>[2x]GPLGSMEGFERELDNIPDTLPDDERLALWKGKLKHYLILSSAGKPIWSRHGDLSLVNSTMGVVQTIISFYEGARNPLLGFTAGKVRFVILIKGPLYFVAISRLRESDAQLRAQLEALYMQILSTLTLPILTNIFAHRPSTDLRGPLQGTESLLASLADSFTKGSPS;>SMTTPVSPSPSGIIPAQLGFLAIYNPALGTTDETLEDQIVYYATASTLSQARRRHRRPRRRDRQRAQSVVKDSRPNAAGATGDSEAVAEDKDPVSKEERHERLRQIGLAQGMVEFAKSFSDGEPVDTIDTEKARVILVEVEEGWWILASIDLTRLPLPQIKTPTSSSAPPPAPNLNPLPPEPAYEYSSREVKPPSLLRADLLRAYDLFLLHHGSSLSSLLASQGRAQLVASLTRFWDHFLATWNVLLHGN[2x];>[2x]GSMSSRKKVLLKVIILGDSGVGKTSLMNQYVNKKFSASYKATIGADFLTREVMVDDRQVTMQLWDTAGQERFQSLGVAFYRGADCCVLVFDVNNAKSFDALDSWRDEFLIQASPRDPENFPFVVLGIKIDVEESKRVISTKRAQTFCQSKGGIPYFETSAKEAINVEEAFQVIARNALMQEESEEFSGDFQDPINIHIENERDGCAC

MC1 has been identified as the GEF for Rab7/Ypt7 and localizes to LEs1216. The sequential inactivation of Rab5 and activation of Rab7 (Ypt7 in yeast), which then serves as marker for LEs, confers membrane identity and directionality during the endosomal maturation process26. Our study shows that MC1 forms a heterotetrameric complex with specific localization domains and a catalytic core that acts through a unique mechanism, thus representing a novel class of RabGEFs. The enzymatic activity of MC1 is mediated entirely by a core complex consisting of the longin domains of Mon1 and Ccz1 plus an extra N-terminal helix of Mon1.

To gain mechanistic insight into MC1 function, we determined the crystal structure of the catalytically active CtMC1core bound to the nucleotide-free CtYpt7–N125I. The structure was refined to 2.5 Å resolution revealing two CtMC1–Ypt7 complexes per asymmetric unit. Mon1 as well as Ccz1 adopt the typical longin domain architecture, with Mon1 harbouring an additional α-helix α0 at the N-terminus (D211 to G220). In the asymmetric unit the C-terminal α-helices α3 of both CtMon1 molecules are swapped such that a dimer of the trimeric CtMC1–Ypt7 complex is formed. The heterodimerization of CtMon1 and CtCcz1 is mainly mediated by the central β-strands of both proteins, which form a continuous β-sheet, and the α-helices α1, which are oriented on top of the β-sheet alongside another in an antiparallel manner. The interface of the MC1 complex with Ypt7 is mainly formed by Mon1 (∼960 Å2) with smaller contributions of Ccz1 (∼450 Å2). An additional interaction interface is formed by the ‘elbow loop' between helices α2 and α3 of Mon1 that interacts with the α3–β5 loop of Ypt7 (∼350 Å2). In the CtMC1–Ypt7 complex, the conformation of the Ypt7 P-loop is identical to the nucleotide-bound form and coordinates a sulfate ion from the crystallization condition at the position that would be occupied by the β-phosphate of GDP or GTP. Interaction with MC1 leads to a dramatic remodelling of the nucleotide-binding pocket of Ypt7. Switch I is moved 18 Å and switch II 8 Å compared with the active conformation observed for ScYpt7 in complex with the GTP analogue GNP (guanosine 5′-[β,γ-imido]triphosphate).>[2x]ADPGTSECSVIGYNAICINRGLHQVPELPAHVNYVDLSLNSIAELNETSFSRLQDLQFLKVEQQTPGLVIRNNTFRGLSSLIILKLDYNQFLQLETGAFNGLANLEVLTLTQCNLDGAVLSGNFFKPLTSLEMLVLRDNNIKKIQPASFFLNMRRFHVLDLTFNKVKSICEEDLLNFQGKHFTLLRLSSITLQDMNEYWLGWEKCGNPFKNTSITTLDLSGNGFKES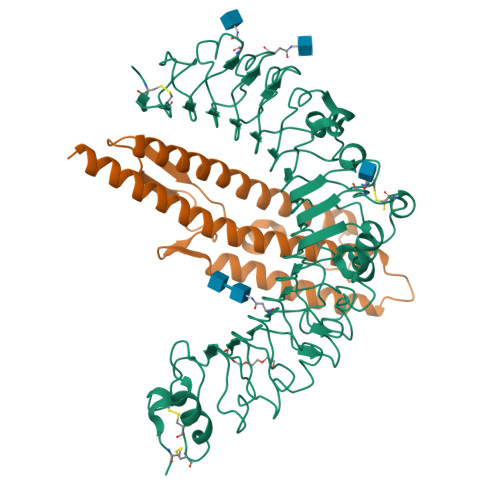MAKRFFDAIAGTKIQSLILSNSYNMGSSFGHTNFKDPDNFTFKGLEASGVKTCDLSKSKIFALLKSVFSHFTDLEQLTLAQNEINKIDDNAFWGLTHLLKLNLSQNFLGSIDSRMFENLDKLEVLDLSYNHIRALGDQSFLGLPNLKELALDTNQLKSVPDGIFDRLTSLQKIWLHTNPWDCSCPRIDYLSRWLNKNSQKEQGSAKCSGSGKPVRSIICPTSASLVPR;>GSAKDPGQIRGLEMASKNSQDGISLIQTAEGALTETHAILQRMRELTVQAGNTGTQQAEDLGAIKDEMDALIEEIDGISNRTEFNGKKLLDGTNSTDGFTFQIGANAGQQLNVKIDSMSSTALGVNALDVTDFAATAFDDQLKSIDTAINTVSTQRAKLGAVQNRLEHTINNLGASGENLTAA[2x]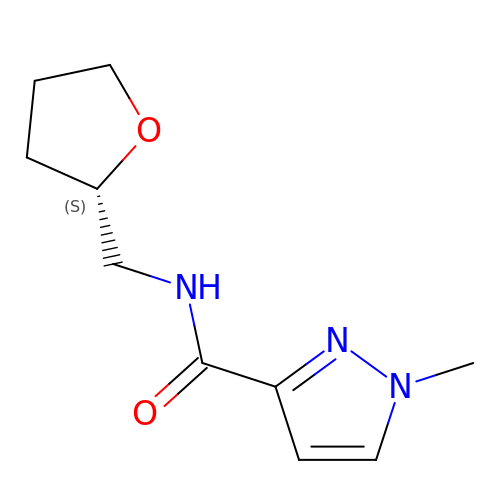1-methyl-N-{[(2S)-oxolan-2-yl]methyl}-1H-pyrazole-3-carboxamide | C10 H15 N3 O2 | WBAZBPMBDLSPCX-QMMMGPOBSA-N>[2x]HHHHHHENLYFQGELKRE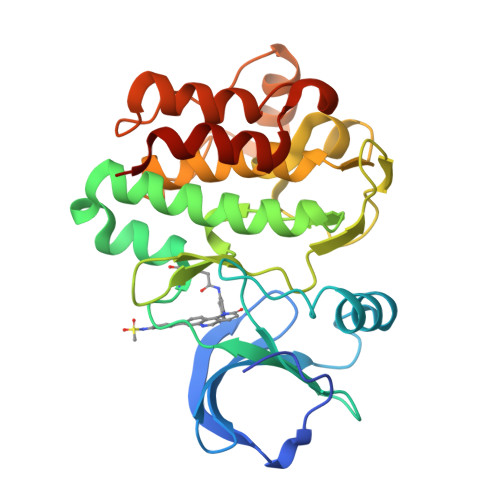EITLLKELGSGQFGVVKLGKWKGQYDVAVKMIKEGSMSEDEFFQEAQTMMKLSHPKLVKFYGVCSKEYPIYIVTEYISNGCLLNYLRSHGKGLEPSQLLEMCYDVCEGMAFLESHQFIHRDLAARNCLVDRDLCVKVSDFGMTRYVLDDQYVSSVGTKFPVKWSAPEVFHYFKYSSKSDVWAFGILMWEVFSLGKMPYDLYTNSEVVLKVSQGHRLYRPHLASDTIYQIMYSCWHELPEKRPTFQQLLSSIEPLREKDKH>CSMAPTYERPAAPVADSWSGAAAQRQGAAIDTLDWKSFIVDAELRRLVDMALDNNRSLRQTLLDIEAARAQYRIQRADRVPGLNAAATGNRQRQPADLSAGNRSEVASSYQVGLALPEYELDLFGRVKSLTDAALQQYLASEEAARAARIALVAEVSQAYLSYDGALRRLALTRQTLVSREYSFALIDQRRAAGAATALDYQEALGLVEQARAEQERNLRQKQQAFNALVLLLGSDDAAQAIPRSPGQRPKLLQDIAPGTPSELIERRPDILAAEHRLRARNADI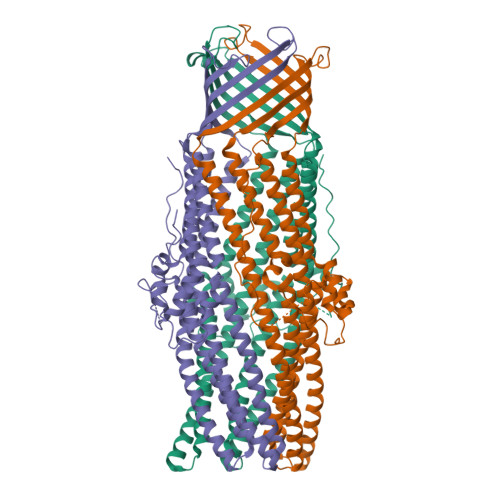GAARAAFFPRISLTGSFGTSSAEMSGLFDGGSRSWSFLPTLTLPIFDGGRNRANLSLAEARKDSAVAAYEGTIQTAFREVADALAASDTLRREEKALRALANSSNEALKLAKARYESGVDNHLRYLDAQRSSFLNEIAFIDGSTQRQIALVDLFRALGGGWDEGRSLVVHRGGRSGSHHHHHH[3x]> GPHMTVAEDKTFQYIRQHHSNFSRIHVLRILPYLSCLTTSDQDRLRATYERWGNQDTLLELFTSLRRRNGWVHSLIGALRACELSGLADEVARIYHS

Recognition of viral RNAs by RLRs leads to the activation of mitochondrial antiviral signaling protein (MAVS; also known as IPS1, VISA and CARDIF). Activated MAVS triggers rapid production of type I interferons and proinflammatory cytokines. It consists of an N-terminal CARD domain, a proline-rich region (PRR) preceding a poorly structured middle segment, and a monotopic transmembrane (TM) domain at the very C-terminus. The N-terminal CARD domain of MAVS is necessary and sufficient for forming active MAVS aggregates.

At the inter-strand interface, the positive and negative charges are alternately distributed at two opposite ends of each CARD subunit, indicating that the inter-strand interaction is mainly electrostatic. The positively charged residues R37 in the 3rd helix (H3), R64 and R65 in the loop between the 4th and 5th helices (H4 and H5) from the CARD in a lower layer (purple in Figure 2B) are in close proximity to the negatively charged residues D23 in the loop between the 1st and 2nd helices (H1b and H2) and E26 in the 2nd helix (H2) of another CARD molecule (cyan in Figure 2B) in the upper layer. E26, R64 and R65 are highly conserved among MAVS molecules from different species, but D23 and R37 are less so. To test the energetic contributions of these charged residues to the stability of the filament and the in vivo MAVS signaling activity, we mutated them individually to an alanine residue or residues with reversed charges. Compared with the wild-type MAVS, which potently induced IFNβ in a dose-dependent manner, point mutations at multiple locations of the inter-strand interface abolished MAVS activity. The gel-filtration profiles (E26R as an example in Figure 2—figure supplement 1A) and the EM images of the negatively stained proteins verified that these mutations impaired the filament formation of the MAVS CARD.>[4x]MEHHHHHHATNLRGVMAALLTPFDQQQALDKASLRRLVQFNIQQGIDGLYVGGSTGEAFVQSLSEREQVLEIVAEEAKGKIKLIAHVGCVSTAESQQLAASAKRYGFDAVSAVTPFYYPFSFEEHCDHYRAIIDSADGLPMVVYNIPALSGVKLTLDQINTLVTLPGVGALKQTSGDLYQMEQIRREHPDLVLYNGYDEIFASGLLAGADGGIGSTYNIMGWRYQGIVKALKEGDIQTAQKLQTECNKVI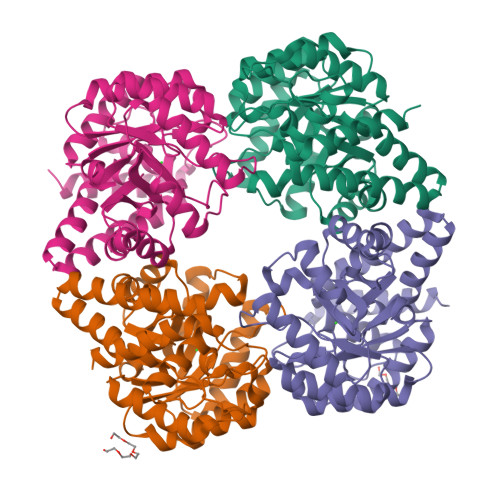DLLIKTGVFRGLKTVLHYMDVVSVPLCRKPFGPVDEKYLPELKALAQQLMQERG6-AMIDINE-2-(4-AMIDINO-PHENYL)INDOLE | C16 H15 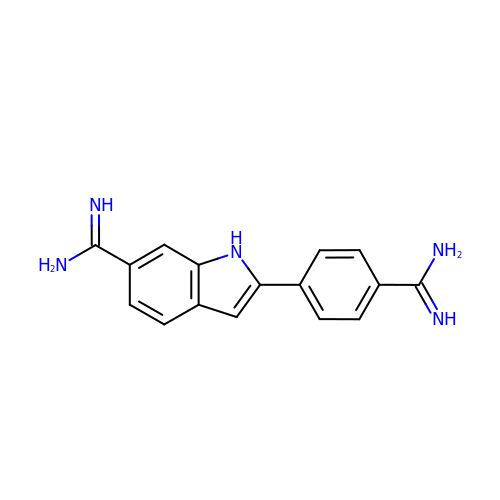N5 | FWBHETKCLVMNFS-UHFFFAOYSA-N>[2x]MIAAQLLAYYFTELKDDQVKKIDKYLYAMRLSDETLIDIMTRFRKEMKNGLSRDFNPTATVKMLPTFVRSIPDGSEKGDFIALDLGGSSFRILRVQVNHEKNQNVHMESEVYDTPENIVHGSGSQLFDHVAECLGDFMEKRKIKDKKLPVGFTFSFPCQQSKIDEAILITWTKRFKASGVEGADVVKLLNKAIKKRGDYDANIVAVVNDTVGTMMTCGYDDQHCEVGLIIGTGTNACYMEELRHIDLVEGDEGRMCINTEWGAFGDDGSLEDIRTEFDREIDRGSLNPGKQLFEKMVSGMYLGELVRLILVKMAKEGLLFEGRITPELLTRGKFNTSDVSAIEKNKEGLHNAKEILTRLGVEPSDDDCVSVQHVCTIVSFRSANLVAATLGAILNRLRDNKGTPRLRTTVGVDGSLYKTHPQYSRRFHKTLRRLVPDSDVRFLLSESGSGKGAAMVTAVAYRLAEQHRQIEETLAHFHLTKDMLLEVKKRMRAEMELGLR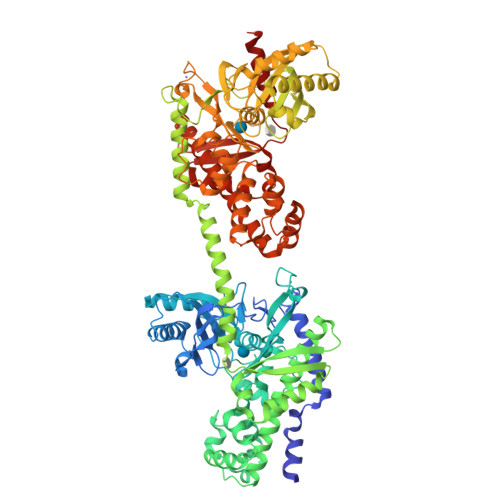KQTHNNAVVKMLPSFVRRTPDGTENGDFLALDLGGTNFRVLLVKIRSGKKRTVEMHNKIYAIPIEIMQGTGEELFDHIVSCISDFLDYMGIKGPRMPLGFTFSFPCQQTSLDAGILITWTKGFKATDCVGHDVVTLLRDAIKRREEFDLDVVAVVNDTVGTMMTCAYEEPTCEVGLIVGTGSNACYMEEMKNVEMVEGDQGQMCINMEWGAFGDNGCLDDIRTHYDRLVDEYSLNAGKQRYEKMISGMYLGEIVRNILIDFTKKGFLFRGQISETLKTRGIFETKFLSQIESDRLALLQVRAILQQLGLNSTCDDSILVKTVCGVVSRRAAQLCGAGMAAVVDKIRENRGLDRLNVTVGVDGTLYKLHPHFSRIMHQTVKELSPKCNVSFLLSEDGSGKGAALITAVGVRLRTE> MPEADRELVSIR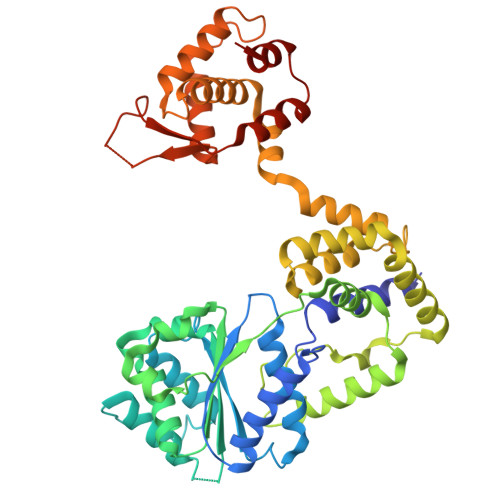RFLKERLQRDYTTLRGYAKERSNVRLLLQRTAEMGESNSLLLLGPRGSGKTTLINSVLADLLPNKSFGENTLIVHLDGNLHTDDRVALKSITVQMQLENAADGKVFGSFAENLAFLLQCLKAGGKHSKSVIFILEEFDLFCAHHNQTLLYNLFDVSQSAQAPICVLGVTCRLDVIELLEKRVKSRFSHRQVFLFPSLRRFEDYVDLCRDLLSLPTGNSLLLAAEKIYNLQNIQSGALYFSRNHFDPGEYGFSPRLRDAWNKQICKVLATQQARSTLQALHDFDISEAYLKNFLFRLVAHLRPQSPHITAEKMAAVGSQFEGDDKIELLCGLSVLELCLIIAIKHHSQIYDRDSFNFEIIYARFSKFAKVSTTMQAVERSIVLKAFEHLRIAELIMPLTGGAGGGVGKVQKEFEMHKLALTYSQIHHCMQRYQALPTEVAQWAQSSLI>DELAFSPPFYPSPWANGQGEWAEAYQRAVAIVSQMTLDEKVNLTTGTGWELEKCVGQTGGVPRLNIGGMCLQDSPLGIRDSDYNSAFPAGVNVAATWDKNLAYLRGQAMGQEFSDKGIDVQLGPAAGPLGRSPDGGRNWEGFSPDPALTGVLFAETIKGIQDAGVVATAKHYILNEQEHFRQVAEAAGYGFNISDTISSNVDDKTIHEMYLWPFADAVRAGVGAIMCSYNQINNSYGCQNSYTLNKLLKAELGFQGFVMSDWGAHHSGVGSALAGLDMSMPGDITFDSATSFWGTNLTIAVLNGTVPQWRVDDMAVRIMAAYYKVGRDRLYQPPNFSSWTRDEYGFKYFYPQEGPYEKVNHFVNVQRNHSEVIRKLGADSTVLLKNNNALPLTGKERKVAILGEDAGSNSYGANGCSDRGCDNGTLAMAWGSGTAEFPYLVTPEQAIQAEVLKHKGSVYAITDNWALSQVETLAKQASVSLVFVNSDAGEGYISVDGNEGDRNNLTLWKNGDNLIKAAANNCNNTIVVIHSVGPVLVDEWYDHPNVTAILWAGLPGQESGNSLADVLYGRVNPGAKSPFTWGKTREAYGDYLVRELNNGNGAPQDDFSEGVFIDYRGFDKRNETPIYEFGHGLSYTTFNYSGLHIQVLNASSNAQVATETGAAPTFGQVGNAS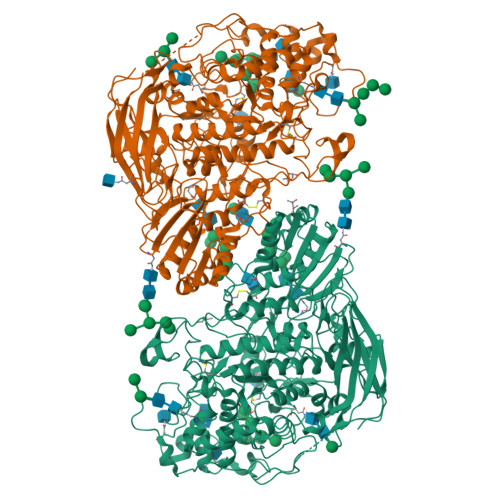DYVYPEGLTRISKFIYPWLNSTDLKASSGDPYYGVDTAEHVPEGATDGSPQPVLPAGGGSGGNPRLYDELIRVSVTVKNTGRVAGDAVPQLYVSLGGPNEPKVVLRKFDRLTLKPSEETVWTTTLTRRDLSNWDVAAQDWVITSYPKKVHVGSSSRQLPLHAALPKVQ[2x]>[2x]ILKELENLSPEEAAHQKAVVETLLQEDPWRVAKMVKSYLQQHNIPQREVVDTTGLNQSHLSQHLNKGTPMKTQKRAALYTWYVRKQR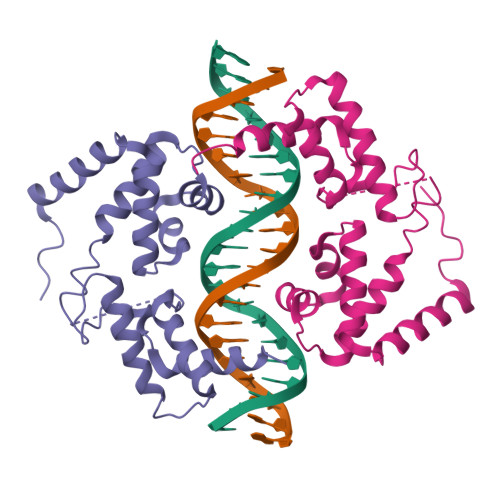EVAQQFTHAGQGGLIEEPTGDELPTKKGRRNRFKWGPASQQILFQAYERQKNPSKEERETLVEECNRAECIQRGVSPSQAQGLGSNLVTEVRVYNWFANRRKEEAFR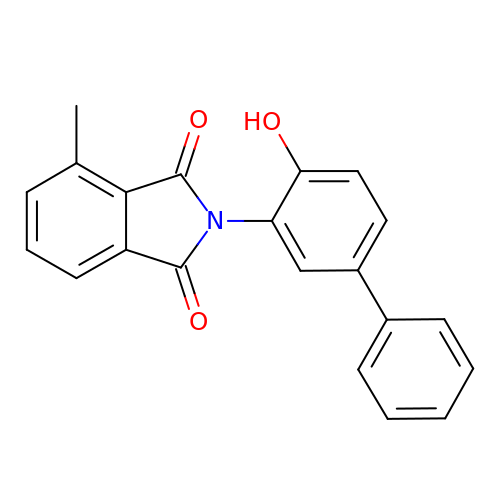2-(4-hydroxybiphenyl-3-yl)-4-methyl-1H-isoindole-1,3(2H)-dione | C21 H15 N O3 | ROMNEYAQUBNRLR-UHFFFAOYSA-N>[2x]MSAFITFEGPEGSGKTTVINEVYHRLVKDYDVIMTREPGGVPTGEEIRKIVLEGNDMDIRTEAMLFAASRREHLVLKVIPALKEGKVVLCDRYIDSSLAYQG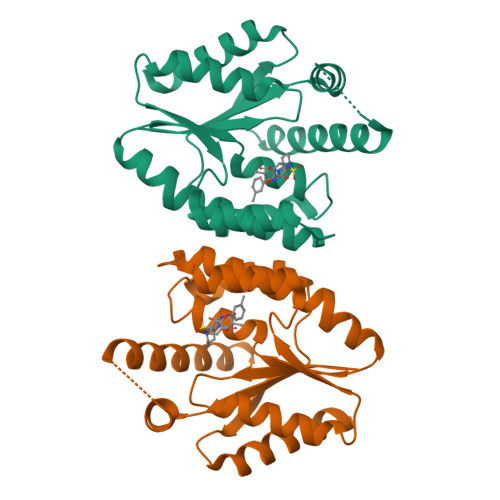YARGIGVEEVRALNEFAINGLYPDLTIYLNVSAEVGRERIIKNSRDQNRLDQEDLKFHEKVIEGYQEIIHNESQRFKSVNADQPLENVVEDTYQTIIKYLEKI> MENLTEMLKGSLEGCVLEIISRRETYGYEITRHLNDLGFTEVVEGTVYTILVRLEK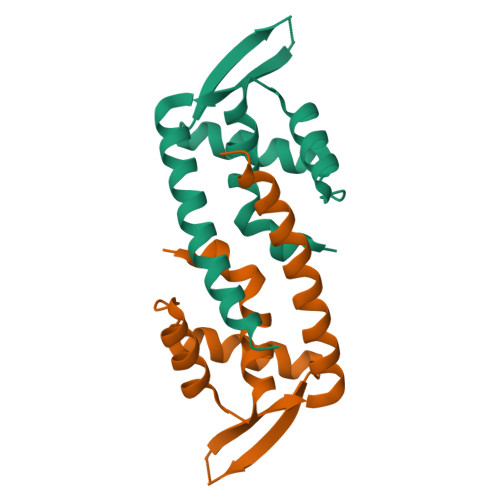KKLVNIEKKPSDMGPPRKFYSLNEAGRQELELFWKKWDFVSSKINVLKSSNSRWSHPQFEK>[2x]GAMSSEMSTICDKTLNPSFCLKFLNTKFASANLQALAKTTLDSTQARATQTLKKLQSIIDGGVDPRSKLAYRSCVDEYESAIGNLEEAFEHLASGDGMGMNMKVSAALDGADT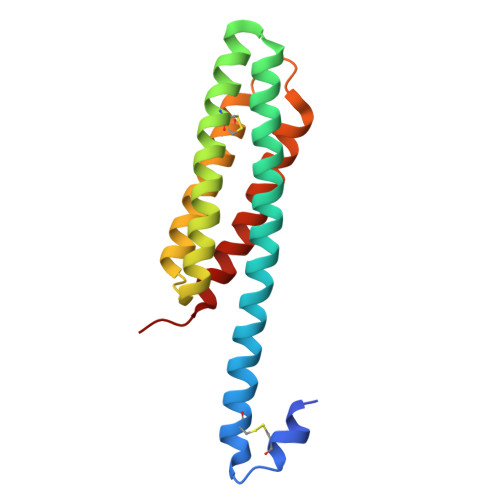CLDDVKRLRSVDSSVVNNSKTIKNLCGIALVISNMLPRN N-[(R)-({[(benzyloxy)carbonyl]amino}methyl)(hydroxy)phosphoryl]-L-leucyl-L-norvaline 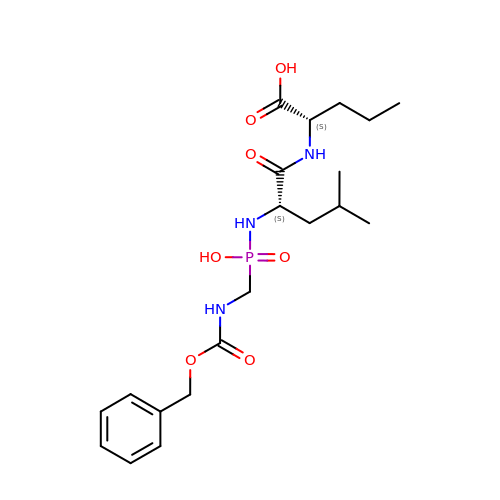| C20 H32 N3 O7 P | NARUKCIBPXPBKJ-IRXDYDNUSA-N>[4x]MLCEIECRALSTAHTRLIHDFEPRDALTYLEGKNIFTEDHSELISKMSTRLERIANFLRIYRRQASELGPLIDFFNYNNQSHLADFLEDYIDFAINEPDLLRPVVIAPQFSRQMLDRKLLLGNVPKQMTCYIREYHVDRVIKKLDEMCDLDSFFLFLHGRAGSGKSVIASQALSKSDQLIGINYDSIVWLKDSGTAPKSTFDLFTDILLMLKSEDDLLNFPSVEHVTSVVLKRMICNALIDRPNTLFVFDDVVQEETIRWAQELRLRCLVTTRDVEISNAASQTCEFIEVTSLEIDECYDFLEAYGMPMPVGEKEEDVLNKTIELSSGNPAT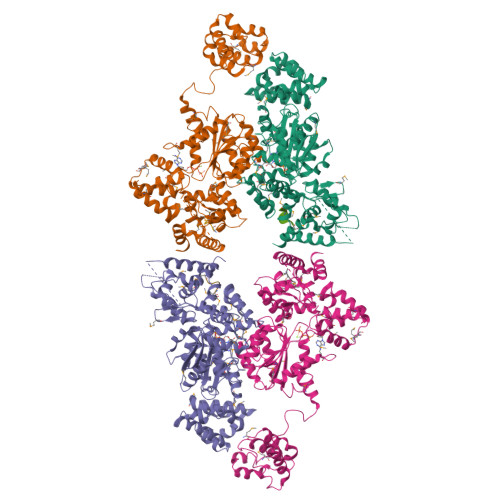LMMFFKSCEPKTFEKMAQLNNKLESRGLVGVECITPYSYKSLAMALQRCVEVLSDEDRSALAFAVVMPPGVDIPVKLWSCVIPVDICSNEEEQLDDEVADRLKRLSKRGALLSGKRMPVLTFKIDHIIHMFLKHVVDAQTIANGISILEQRLLEIGNNNVSVPERHIPSHFQKFRRSSASEMYPKTTEETVIRPEDFPKFMQLHQKFYDSLKNFACC;>[4x]PMFNFMGC> GPHMAQGTLIRVTPEQPTHAVCVLGTLTQLDICSSAPEDCTSFSINASPGVVVDIAHSPPAKKKSTGSSTWPLDPGVEVTLTMKAASGSTGDQKVQISYYGPKTPPVKA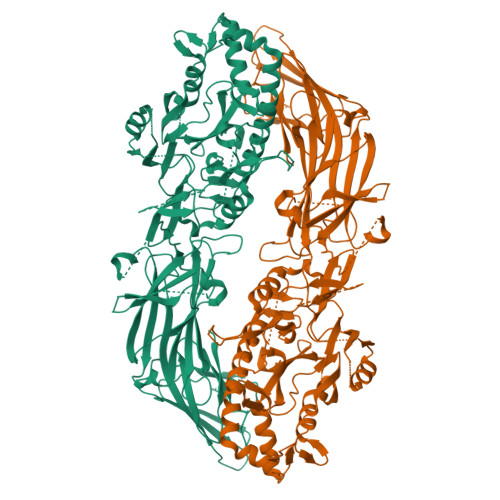LLYLTAVEISLCADITRTGKVKPTRAVKDQRTWTWGPCGQGAILLVNCDRDNLESSAMDCEDDEVLDSEDLQDMSLMTLSTKTPKDFFTNHTLVLHVARSEMDKVRVFQATRGKLSSKCSVVLGPKWPSHYLMVPGGKHNMDFYVEALAFPDTDFPGLITLTISLLDTSNLELPEAVVFQDSVVFRVAPWIMTPNTQPPQEVYACSIFENEDFLKSVTTLAMKAKCKLTICPEEENMDDQWMQDEMEIGYIQAPHKTLPVVFDSPRNRGLKEFPIKRVMGPDFGYVTRGPQTGGISGLDSFGNLEVSPPVTVRGKEYPLGRILFGDSCYPSNDSRQMHQALQDFLSAQQVQAPVKLYSDWLSVGHVDEFLSFVPAPDRKGFRLLLASPRSCYKLFQEQQNEGHGEALLFEGIKKKKQQKIKNILSNKTLREHNSFVERCIDWNRELLKRELGLAESDIIDIPQLFKLKEFSKAEAFFPNMVNMLVLGKHLGIPKPFGPVINGRCCLEEKVCSLLEPLGLQCTFINDFFTYHIRHGEVHCGTNVRRKPFSFKWWNMVP>MAEPWGNELASAAARGDLEQLTSLLQNNVNV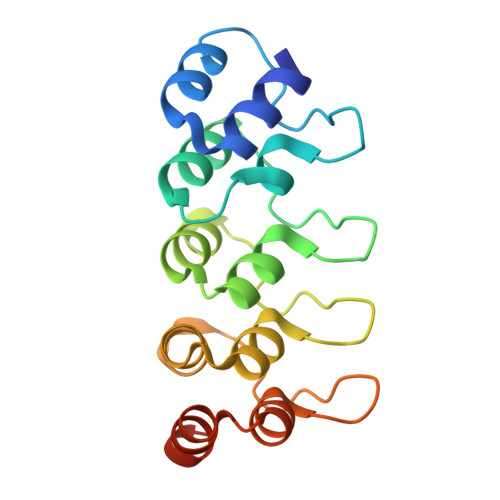NAQNGFGRTALQVMKLGNPEIARRLLLRGANPDLKDRTGFAVIHDAARAGQLDTLQTLLEFQADVNIEDNEGNLPLHLAAKEGHLRVVEFLVKHTASNVGHRNHKGDTACDLARLYGRNEVVSLMQANGAGGATNLQ[2x]1-(3-methoxyazetidine-1-sulfonyl)pyrrolidine 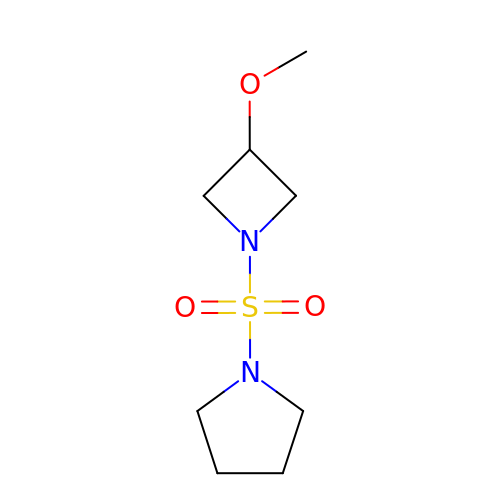| C8 H16 N2 O3 S | KONUKKZPOYOKNK-UHFFFAOYSA-N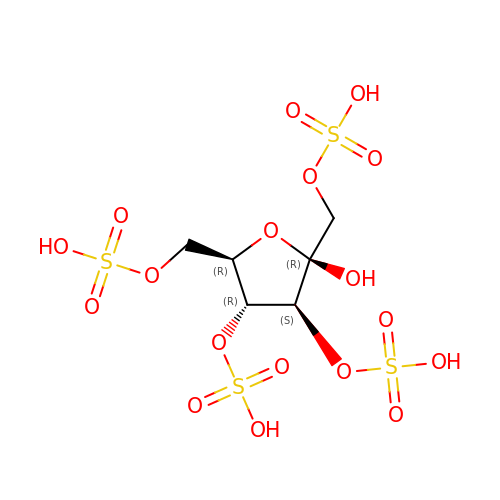1,3,4,6-tetra-O-sulfo-beta-D-fructofuranose | C6 H12 O18 S4 | UCVVRDOLNRDLDM-ARQDHWQXSA-N Recent proteomic studies have identified a novel HDAC1/2 complex in Homo sapiens and Caenorhabditis elegans called the MiDAC complex. In this paper, we show that DNTTIP1 forms a stoichiometric complex with HDAC1 and the ELM2-SANT domain from MIDEAS. In conclusion, we have shown that DNTTIP1 is a dimeric protein required for the stable assembly of the cyclin A associated MiDAC complex. In addition to contributing to the assembly of this complex, DNTTIP1 also mediates a chromatin-binding activity that is likely to be important for substrate presentation to the active catalytic site of HDAC1.

Human DNTTIP1 (56–147) crystallized with six molecules within the asymmetric unit. The structure was solved at 2.1 Å resolution using MAD phasing with seleno-methionine substituted protein. It was immediately clear in the electron density that the protein was arranged in the asymmetric unit as three dimers. Each monomer consists of a long amino-terminal helix divided into three by two distinct kinks. Carboxy-terminal to this long helix, the peptide chain folds back on itself leading into a second, shorter helix arranged at ∼60° to the central portion of the longer helix. The dimer is arranged such that the longer helices in the two monomers lie anti-parallel to each other and form a saddle into which the two shorter carboxy-terminal helices are packed together, also in an anti-parallel orientation. This arrangement results in a large buried surface between the two monomers of 4083 Å2. Remarkably, this represents 69% of the whole surface of the monomer. The core of the interface between the monomers consists entirely of non-polar amino acid side chains. The Dali protein structure comparison server identifies no structures that are significantly similar to the DNTTIP1 dimerization domain suggesting that this is a novel fold.

>MTTSFTDPAISMDLLRAVLQPSINEEIQTVFNKYMKFFQKAALNVRDNVGEEVDAEQLIQEACRSCLEQAKLLFSDGEKVIPRLTHELPGIK[6x]> SAAANDVNYSFDEAVSMQQGKGIVQTKEEDGKFVEANNNEIAKAMTISHKDNDMKYMDITEKVPMSESEVNQLLKGKGILENRGKVFLEAQEKYEVNVIYLVSHALVETGNGKSELAKGIKDGKKRYYNFFGIGAFDSSAVRSGKSYAEKEQWTSPDKAIIGGAKFIRNEYFENNQLNLYQM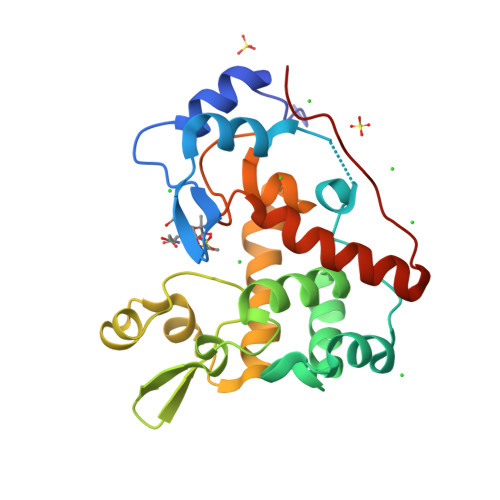RWNPENPAQHQYASDIRWADKIAKLMDKSYKQFGIKKDDIRQTYYK> MRHPIPDYLASLVTELGAVNPGETAQYIPVLAEADPDRFGIALATPTGRLHCAGDADVEFTIQSASKPFTYAAALVDRGFAAVDRQVGLNPSGEAFNELSLEAESHRPDNAMINAGALAVHQLLVGPEASRKERLDR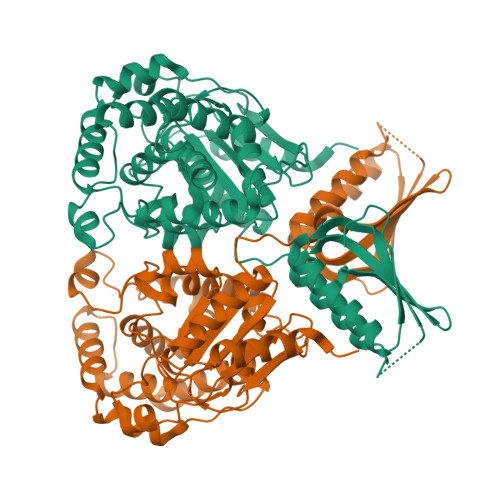AVEIMSLLAGRRLSVDWETYESEMAVSDRNLSLAHMLRSYGVLQDSAEEIVAGYVAQCAVLVTVKDLAVMGACLATGGIHPMTGERMLPSIVARRVVSVMTSSGMYDAAGQWLADVGIPAKSGVAGGVLGALPGRVGIGVFSPRLDEVGNSARGVLACRRLSEDFRLHLMDGDSLGGTAVRFVEREGDRVFLHLQGVIRFGGAEAVLDALTDLRTGAEKPGTGWDAAVYPRWQEAAADRAALSAATGGGAVHEAAAAAARDENDGPIRTVVLNLARVDRIDDVGRRLIAEGVRRLQADGVRVEVEDPERILPLEEAGAH>[4x]MKLSGVEL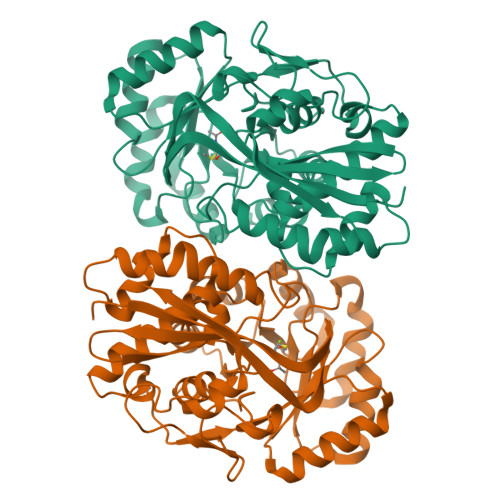RRVQMPLVAPFRTSFGTQSVRELLLLRAVTPAGEGWGECVTMAGPLYSSEYNDGAEHVLRHYLIPALLAAEDITAAKVTPLLAKFKGHRMAKGALEMAVLDAELRAHERSFAAELGSVRDSVPCGVSVGIMDTIPQLLDVVGGYLDEGYVRIKLKIEPGWDVEPVRAVRERFGDDVLLQVDANTAYTLGDAPQLARLDPFGLLLIEQPLEEEDVLGHAELARRIQTPICLDESIVSARAAADAIKLGAVQIVNIKPGRVGGYLEARRVHDVCAAHGIPVWCGDMIETGLGRAANVALASLPNFTLPGDTSASDRYYKTDITEPFVLSGGHLPVPTGPGLGVAPIPELLDEVTTAKVWIGS> GPMQQANLGDGVATARLLSRSDWGARLPKSVEHFQGPAPYVIIHHSYMPAVCYSTPDCMKSMRDMQDFHQLERGWNDIGFSFGIGGDGMIYTGRGFNVIGAHAPKYNDKSVGIVLIGDWRTELPPKQMLDAAKNLIAFGVFKGY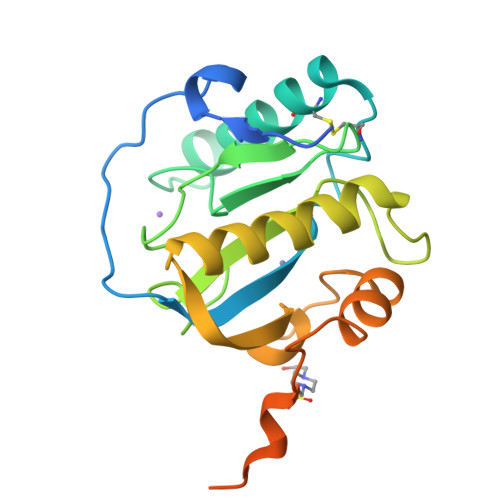IDPAYKLLGHRQVRDTECPGGRLFAEISSWPHFTHINDTEGVSSTTAPVVPHVHPQAAAPQKPHQSPPAAPKV>AQTVPYGIPLIKADKVQAQGFKGANVKVAVLDTGIQASHPDLNVVGGASFVAGEAYNTDGNGHGTHVAGTVAALDNTTGVLGVAPSVSLYAVKVLNSSGSGSYSGIVSGIEWATTNGMDVINMSLGGASGSTAMKQAVDNAYARGVVVVAAAGNSGSSGNTNTIGYPAKYDSVIAVGAVDSNSNRASFSSVGAELEVMAPGAGVYSTYPTNTYATLNGTSMASPHVAGAAALILSKHPNLSASQVRNRLSSTATYLGSSFYYGKGLINVEAAAQ[3x];> APCPHTYKPVCGANGEVYDNECFLNKAGIEPAESWETCRGHELCPSVCTEEYDPVCVEGKIYGNRCMQSHFCGKV

During our recent work on subtractive ESTs (expressed sequence tags) from the Carcinoscorpius rotundicauda that was infected with Pseudomonas aeruginosa, two isoforms of the non-classical Kazal-type inhibitor, CrSPI, each of 9.3 kDa, were discovered. Earlier, we have proposed that CrSPI-1 may act as an “on-off” regulatory switch in the modulation of antimicrobial activities while maintaining homeostasis of host proteases. CrSPI-1 has been proposed to regulate the serine protease-driven antimicrobial defense during the acute phase of infection while maintaining homeostasis under normal physiological conditions.

Here, we report the crystal structure of the two-headed non-classical Kazal-type group I inhibitor CrSPI-1 in complex with its cognate protease, subtilisin, at a stoichiometric ratio of 1∶2 (CrSPI-1 to subtilisin) and refined up to 2.6 Å resolution. There were three subtilisin molecules and one CrSPI-1 molecule in the asymmetric unit. Each CrSPI-1 molecule interacted with two subtilisin molecules, i.e., domain 1 and domain 2 of CrSPI-1 interacted with two independent subtilisin molecules. The third subtilisin molecule of the asymmetric unit was not in a complex with CrSPI-1. The three subtilisin molecules of the asymmetric unit were identical with an rmsd of 0.1 Å in a pairwise superimposition of 274 Cα atoms. This indicates that there was no significant conformational change of subtilisin molecules upon complex formation with the CrSPI-1 molecule. The CrSPI-1 molecule comprises two domains: domain 1 from Cys1 to Glu40 and domain 2 from Leu41 to Leu83. Both domains adopted similar secondary structures (domain 1 β1↑β2↓α1β3↑ and domain 2 β4↑β5↓α2). The reactive site loops of both domains of CrSPI-1 occupy the substrate binding pockets of subtilisin. The reactive site loop (RSL) of domain 1 of CrSPI-1 (Cys1 to Lys6) binds at the active site region of subtilisin from P3 (Cys1) to P3′ (Lys6) in a substrate-like manner. In domain 2 of CrSPI-1, Glu49 takes the position of His3 in the P1 pocket of domain 1 and makes 8 (73%) of the 11 total hydrogen bonding contacts with subtilisin.In eukaryotes, wobble uridines are modified by Elongator, a large and highly conserved macromolecular complex. Elongator consists of two subcomplexes, namely Elp123 containing the enzymatically active Elp3 subunit and the associated Elp456 hetero-hexamer. The Elongator complex harbors two copies of each of its six subunits, namely Elongator proteins 1–6 (Elp1–Elp6). Decreased levels of wobble uridine modifications lead to ribosome pausing, incorrect protein folding and consequently trigger intracellular protein aggregation and proteotoxic stress.

As we observed unbound ring-shaped Elp456 particles in one of our datasets, we also determined the cryo-EM structure of free full-length ScElp456 at 3.7 Å overall resolution. The newly obtained structures of full-length Elp456 are almost identical to the truncated crystal structure of the Elp456 subcomplex. The structure confirms that Elp456 contains two copies of Elp4, Elp5 and Elp6, forming a symmetric dimer of trimers. However, the N- and C-terminal extensions of Elp4 and Elp5 (including a small predicted domain at the C-terminus of Elp5 (85)) remain flexible also in the fully assembled complex.

>MSFRKRGEILNDRGSGLRGPLLRGPPRTSSTPLRTGNRRAPGNVPLSDTTARLKKLNIADESKTKMGLDSSHVGVRPSPATSQPTTSTGSADLDSILGHMGLPLGNSVLVEEQSTTEFHSILGKLFAAQGIVHNRISDSSADKTRNGDTHVIVLSLNQMFAKELPGIYKGSRKQMKKNLISEEESKVTVQNLNETQRSTPSRYKDLKIAWKYKLADEKRLGSPDRDDIQQNSEYKDYNHQFDITTRLMPAPIASELTFIAPTQPVSTILSQIEQTIKRNDKKLIRIVIPSLLHPAMYPPKMFESSEIIGLMHGVRSLVKKYYERVVLFASISIDIITPPLLVLLRNMFDSVINLEPFNQEMTEFLERVYKSQPGKIQHGLVHILKLPVFTDRGEMRVLKSEWAFKNGRKKFEIEQWGIPVDDAEGSAASEQSHSHSHSDEISHNIPAKKTKISLDY[2x];>[2x]MASSSHNPVILLKRILSLTESSPFILCLDSIAQTSYKLIQEFVHQSKSKGNEYPIVYISFETVNKPSYCTQFIDATQMDFVHLVKQIISYLPAATATQAKKHMVIIDSLNYISTEYITRFLSEIASPHCTMVATYHKDIKDENRTVIPDWNNNYPDKLTLLQFMATTIVDIDVVLTGTLDTEEVSELLNEFRIPRGLNNDIFQLRLVNKRKSGRSLEYDFIVNSNTHEYELLSTTKQEEESSSNGLETPEMLQGLTTFNLGTSNKQKLAKDQVALPFLEAQSFGQGGAIVYEYEKDDDYDEEDPYEDPF;>[2x]MGSVQRQDLVLFSDQSVLPAHFFQDSNSHNLFFITHQSCTQPLWMINALVETHVLGSPSSLNESSSSMLPSSTRSHAVLASFIHEQNYFTNSLNKLKIPSNNYNVLDFLSDFIVNNIHNKPRDKILSDVLAKFSAAIQNNPTDTIVIIEQPELLLSLVSGLTCSELNNKFITPLLRQCKVLIIVSNSDIFNIDEYDASVHSSNLQNFYKSSFIKSMINLNLNPLKTGFAKDVTGSLHVCRGGAPIATSNTSLHVVENEYLYLNEKESTKLFYR>[2x]GMSNKKLIINADDFGYTPAVTQGIIEAHKRGVVTSTTALPTSPYFLEAMESARISAPTLAIGVHLTLTLNQAKPILPREMVPSLVDEAGYFWHQSIFEEKVNLEEVYNEWDAQIISFMKSGRRPDHIDSHHNVHGKNKKLLGVALALARKYQLPLRNASRSIETKDYLELYQDVRTPDEMLYQFYDKAISTE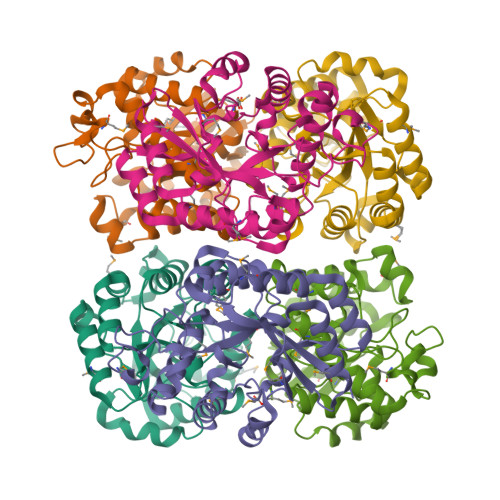TILQLLDMVVCSEGEVFEINCHPAFIDTILQNQSGYCMPRIREVEILTSQEVKEAIEERGILLANYESLAM> MNMYKWVPESIRDSGEGQPSYSNNGDYAPSGPWVAAGIHTMPQSLRDSMRNSIMVTAQARRDVIGPEWGPDGRFTGYASVIGTPDPKPADIVNKFTVERRPVSNGNFQQRVKAGDIVVAPYTSDGKITVKLVAGQKDISSTPDYDYRIDSSLASSAGFVVAGERWYYTKRHFIIPRYFQNWRMRRRKYVTGWVMPTFYSPKEIFNRLKDSLVPDTGLVTQVWADNNTKRMDFLTAMAEIPQTLSSFLDALGYLGSLIKDFKRRRFFLNKAHQRIRNKLGVSFAERRSQIVSKYDRKIASARKPAIIVKLRQRKEKALKALDKMRVREEKKMIREFATQAASLWLSFRYEIMPLYYQSQDVLDVIANSTSEFMTSRDFVAKAINIGIPLEWNLDQENLVSQPRHNVMVKSKLSPENNIGKTLSVNPFTTAWELLTLSFVVDWFVNFGDVIAG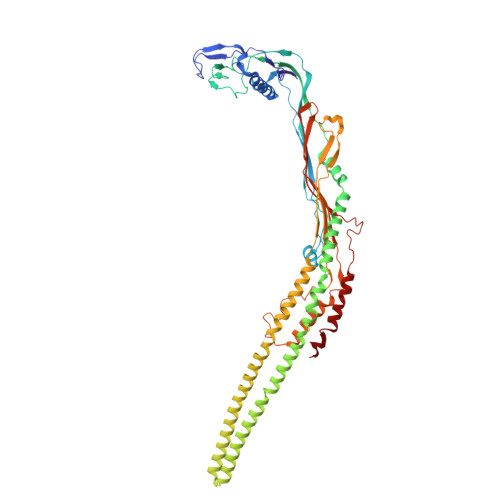FTGGYSDDSGATASWRFDDKKVFHLKNIPSAMVIVDINFYTRQVIDPRLCGGLAFSPKLNLFRYLDAMSLSWNRSRLKISRAT> MILAKVTGHVVATQKCDELRGSNLLLI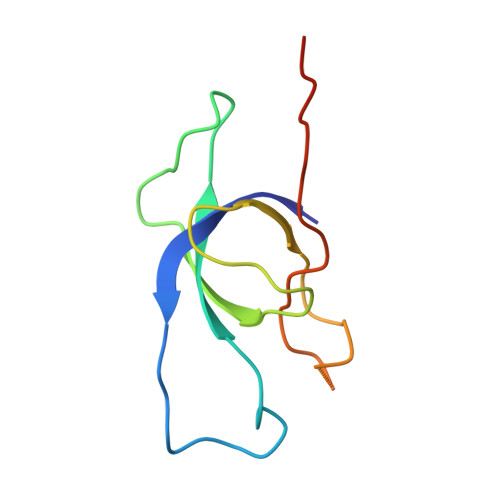TRLDDKQQPMKDQTWVAVDNVGAGMHDIVLAEEYFALNKDRYKAMSVVAIVEKVFRDTEQE> UUCUGCUGCUGAA;> UUCUGCAGCUGAA

Secondary structures formed by expanded CUG RNA are involved in the pathobiology of myotonic dystrophy type 1. Of these repeats, CUG repeat RNA expansion in the 3′-untranslated region of dystrophia myotonica protein kinase mRNA has been shown to play an important role in the pathogenesis of DM1 (24, 25). The expanded CUG RNA forms a hairpin structure and binds the muscleblind like splicing regulator 1 (MBNL1) protein, resulting in splicing defects in the insulin receptor and muscle main chloride ion-related pre-mRNAs. The two RNA duplexes exhibit end-to-end stacking to generate infinite pseudocontinuous CUG helices, which resemble the stem structure of stem-loops known to form in long CUG repeats.

We also solved another crystal structure containing two U–U mismatches and a A–U Watson–Crick pair in the center at a resolution of 1.58 Å that similarly shows a duplex in the asymmetric unit and is referred to as M2 duplex. The sum of roll angles at the central base pair steps of the M3 and M2 duplexes is 13° and 17°, respectively, indicating a sharp bending of the RNA toward the major groove. Interestingly, the helical twist at the three U–U mismatch sites in the M3 duplex has larger values (average = 26.3 ± 1.0°) compared with those in M2 (average = 21.1 ± 0.5°). In the M2 crystal, the λ-angle showed more variations with lower values of 26.8 ± 4.5° and 56.7 ± 1.5°, respectively, indicating that these U–U mismatches are more inclined toward the minor groove compared with those in the M3 structure. In the M2 duplex, the hydrogen bonds of U4–U23 and U10–U17 mismatches with the water molecules are 2.5 Å and 2.8 Å in the minor groove and 3.1 Å and 3.5 Å in the major groove, respectively. Therefore, upon replacing the central U7-U20 mismatch with U7-A20 Watson-Crick base pair, the λ angles are about 58° and 59.9°, respectively. In contrast, the U7–A20 formed two hydrogen bonds with a lower base pair opening of about 6°. Compared with the spectra containing A–U Watson–Crick base pairing, the differences in CD intensity suggested higher levels of distortions in the CUG RNA duplex with lower stability.> LLPVKYCKMRIFSGSTAAAPEEEPFEVWLEQATEIAKEWPIPEAEKKRWVAESLRGPALDLMHIVQADNPSISVGECLEAFKQVF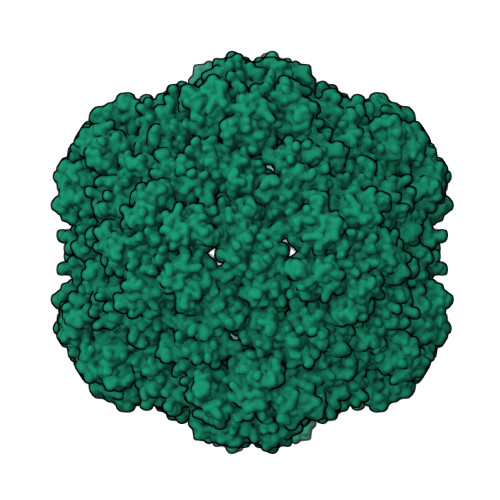GSTESRRTSQVKYLRTYQQEGEKISAYVLRLETLLRRAVEKRAIPRNIADQVRLEQVMAGANLGNVLWCRLQELKDQGPLPTFLQLMKVIREEEE>MAPLENNYNESLNKSKDAIDDKTWSKLFPSIVSDPDRSSNFMIRAIYVVFSAVLRQRNILEKEYFSK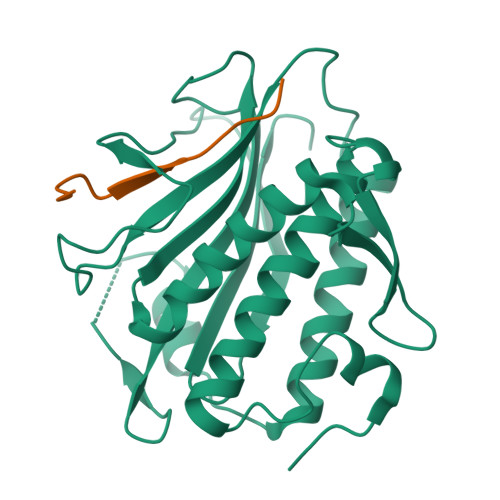NYITENLSCMTLSFKNLRAHQIAQLLRAAGDATKDGFLKEISLVVTEHDGDVEAIEVFSMKFIYFENGGVVARLSTDNNDQEDPHFAELAQLRYEGAESVRDQMVTIVRSVQFLCTKVLEPLPAEFTANFRLKYTNDAPSNFRIDGFDDSSTFYTLPDGIQSVTIGHLRPGHHAAHMQCWSKSMSD[2x];>SNARDSPYGLSQGITKKNKD[2x]Curiously, the suppressor of copper sensitivity C proteins (ScsCs), which are part of the bacterial copper-resistance response, share structural and functional similarities with DSB oxidase and isomerase proteins, including the presence of a catalytic thioredoxin domain. Here, the structure and function of Caulobacter crescentus ScsC (CcScsC) have been characterized. It is shown that CcScsC binds copper in the copper(I) form with subpicomolar affinity and that its isomerase activity is comparable to that of Escherichia coli DsbC, the prototypical dimeric bacterial isomerase. Using mass photometry and small-angle X-ray scattering (SAXS) the protein is demonstrated to be trimeric in solution, like PmScsC, and not dimeric like EcDsbC.

For our structural studies, we used a variant of CcScsC in which the second residue Cys2 is mutated to Ser (CcScsC C2S). One possible explanation for this is that CcScsC wt may form a disulfide bond between the N-terminal cysteines at the high concentration required for crystallization (above 100 mg ml−1, well above physiological levels) and this may interfere with the crystallization process. Replacing Cys2 with Ser in the C2S variant does not affect the disulfide isomerase activity or trimerization of the protein. The crystal structure of CcScsC, solved to a resolution of 2.63 Å, confirms that the protein is trimeric and that the trimer is formed through the interaction of the N-terminal regions of three protomers. The α-helix joins the globular domain of the protein at Tyr52. The globular domain of the CcScsC C2S protomer is a typical thioredoxin fold with two catalytic cysteines (positions 81 and 84; pink sticks in Fig. 6) in close proximity to a cis-Pro motif (Thr191–cis-Pro192). In the unit cell, six protomers are organized by crystallographic symmetry into two trimers. Each trimer is formed from the interaction of the N-terminal α-helical regions of three protomers. While we captured a single conformation of CcScsC C2S in the crystal structure, the comparison between the scattering profiles predicted from the crystal structure and the experimental SAXS data provides strong evidence that the protein trimer can sample multiple conformational states in solution.

> MSDQSKPDKAFGEKVRAYLLEHPEVLMEASQKLQEKQAAQQAVSSQKAIGEYRQAIERDPRDIVINPAGTITVTEFFDYRCGYCRQATPAVLELVQKNPDIRLVLKDFVIFGNDSEAAARIALGAKDQGKSLELHKALMAENALDARGALRIAERLGIDMDKAKAVGESQAITQHLADTDALARALNLSGTPAFIVGDTLVPGADIDALKLAIEQTRAARAKAGLEENLYF> ARLGARPCGLRELE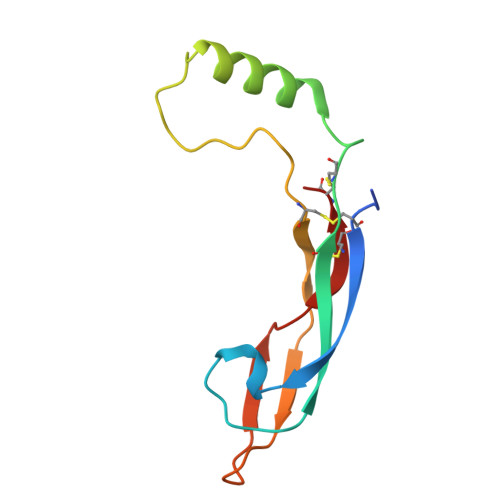VRVSELGLGYASDETVLFRYCAGACEAAARVYDLGLRRLRQRRRLRRERVRAQPCCRPTAYEDEVSFLDAHSRYHTVHELSARECACV> GGAKKNVQDAEGQAEAGGNAPSGYLMPAISANNFCGDFTTMTPDYGYLMPEKGLFLKMHDIRGAYGINIYTYVMDGDNIQCTPGHFVMIVPRGGDKLEITIKKSSMKNTPSFTFIPTPDCENSAYVA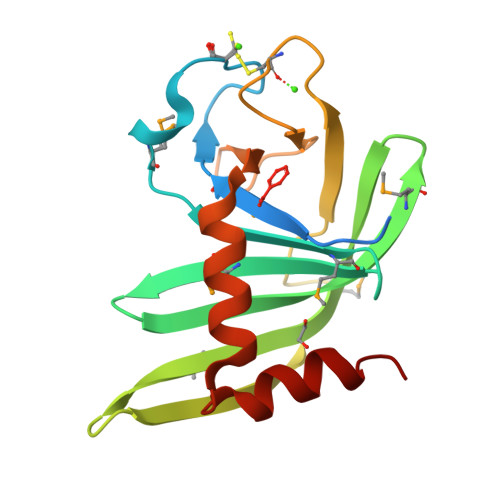TEKVAGKYYYLCGDAEARYKFEDLFEDERCAEFKNLVDNYGK>SQKVEKTVIKNETGTISISQLNKNVWVHTELGSFNGEAVPSNGLVLNTSKGLVLVDSSWDDKLTKELIEMVEKKFQKRVTDVIITHAHADCIGGIKTLKERGIKAHSTALTAELAKKNGYEEPLGDLQTVTNLKFGNMKVETF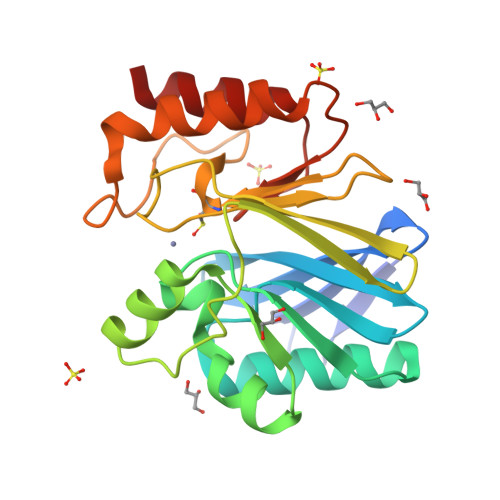YPGKGHTEDNIVVWLPQYNILVGGCLVKSTSAKDLGNVADAYVNEWSTSIENVLKRYRNINAVVPGHGEVGDKGLLLHTLDLLK[2x]> MLRRTVCVQHYRAKLELDRIRSMLRGRARLERKVGLKRLFFLMRTQTRYRVEQQAHWERAIVRKNVDSAAREHGTGWQHLRNELGRQNVMLLPRSQQLLAQYEPLAFRAVVELCASRIPPPPPPVVASVPEESYTLWPPASHDNSECASTDGSDAPHGQQQSLSHPAARVELRCGVERVLRRGPSGLGNNVNELIDA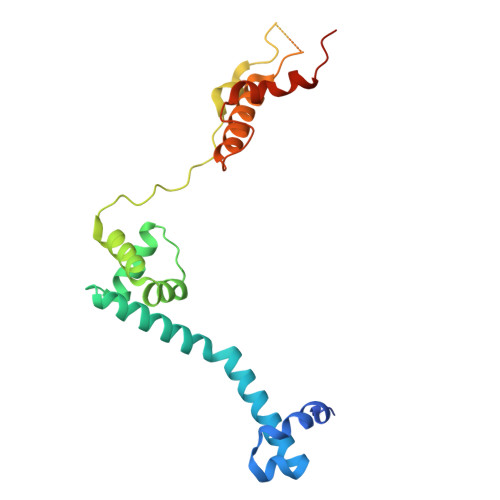WKEFDVSPLRKGEVNK The LASV glycoprotein complex (GPC) mediates viral entry and is the sole target for neutralizing antibodies. In its mature, native form, GPC is a trimer of heterotrimers comprised of the receptor-engaging subunit GP1; the transmembrane-spanning subunit GP2, which contains the GPC’s fusion peptide at its N terminus; and the stable signal peptide (SSP), which remains non-covalently complexed near the membrane-proximal region of GP2 post-cleavage. The GPC is expressed as a single polypeptide precursor before being proteolytically processed by signal peptidase (SPase)21 followed by site-1 protease (S1P). We present the development and characterization of prefusion-stabilized, trimeric GPCs of LASV lineages II, V, and VII, revealing structural conservation despite sequence diversity.

We focus on LASV lineages of public health concern including lineage II, one of the most common lineages that circulates widely in southern Nigeria; lineage V, which circulates in Mali and has decreased pathogenicity compared with lineage IV; and lineage VII, a newly described lineage isolated from a nosocomial infection in Togo with comparable pathogenicity to lineage IV. The resulting soluble constructs feature sequences of circulating lineages II (LII; strain NIG08-A41), V (LV; strain Soromba-R), and VII (LVII; strain Togo/2016/7082). Combined, these approaches enabled us to determine the structures of GPC in a reproducible manner and yielded structures of LIV, LII, LV, and LVII GPC trimers at resolutions of 3.8, 3.7, 3.7, and 3.1 Å, respectively. LII, LV, and LVII each have an additional PNGS at residue N271 or N272, though this site is uniformly unoccupied. Similarly, when comparing the GPCs of diverse lineages, we observe high structural homology. Using the prototypical LIV GPC as reference, we note RMSDs for pruned and all sequence-aligned pair as follows: 0.78 and 1.9 (LII), 0.85 and 2.0 (LV), and 0.73 and 2.4 Å (LVII). The main differences among the GPC lineages are found in flexible loops, most notably the loop (residues 166–181) extending from the β7 sheet prior to the α3 helix. This observed heterogeneity is derived from areas in the EM map of poorer local resolution, insinuating greater flexibility of the residues in these regions. Consequently, these differences may not represent physiologically important conformational epitopes for LII, LV, and LVII GPCs.

>[3x]LIYKGSYELQTLELNMETLNMTMPLSCTKNSSHHYIRVGNETGLELTLTNTSIINHKFCNLSDAHKRNLYDHALMSILSTFHLSIPNFNQYEAMSCDFNGGKISVQYNLSHAYAVDAAEHCGTVANGVLQTFMRMAWGGSYIALDSGCGNWDCIMTSYQYLIIQNTTWEDHCQFSRPSPIGYLGLLSQRTRDIYIS;>GTFTWTLSDSEGNETPGGYCLTRWMLIEAELKCFGNTAVAKCNEKHDEEFCDMLRLFDFNKQAIQRLKSPAQMSIQLINKAVNALINDQLIMKNHLRDMMCIPYCNYSKYWYLNHTSSGRTSLPKCWLVSNGSYLNETHFSDDIEQQADNMITEMLQKEYIDRQG[3x]>MSRPRKRLAGTSGSDKGLSGKRTKTENSGEALAKVEDSNPQKTSATKNCLKNLSSHWLMKSEPESRLEKGVDVKFSIEDLKAQPKQTTCWDGVRNYQARNFLRAMKLGEEAFFYHSNCKEPGIAGLMKIVKEAYPDHTQFEKNNPHYDPSSKEDNPKWSMVDVQFVRMMKRFIPLAELKSYHQAHKATGGPLKNMVLFTRQRLS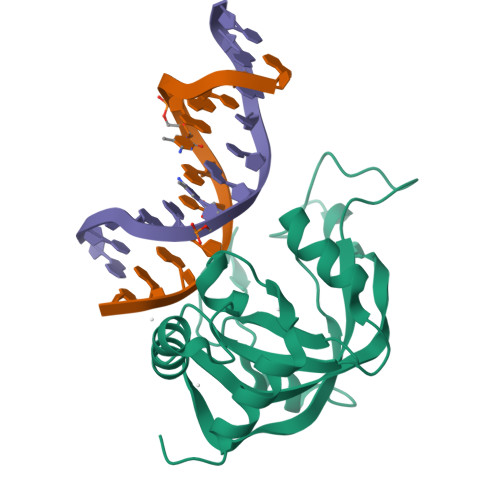IQPLTQEEFDFVLSLEEKEPS[2x]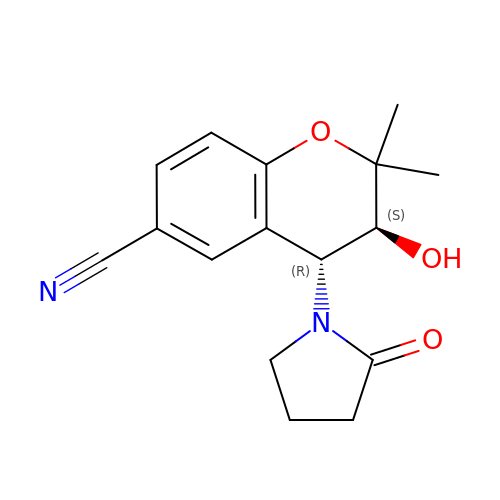(3S,4R)-2,2-dimethyl-3-oxidanyl-4-(2-oxidanylidenepyrrolidin-1-yl)-3,4-dihydrochromene-6-carbonitrile | C16 H18 N2 O3 | TVZCRIROJQEVOT-CABCVRRESA-N>[2x]HMLPKDFQWGFATAAYQIEGAIDKDGRGPSIWDTFCAIPGKIADGTSGVTACDSYNRTAEDIALLKSLGAKSYRFSISWSRIIPKGGRDDPVNQLGIDHYAQFVDDLLEAGITPFITLFHWDLPEELHQRYGGLLNRTEFPLDFENYARVMFKALPKVRNWITFNEPWCSAILGYGSGTFAPGRQS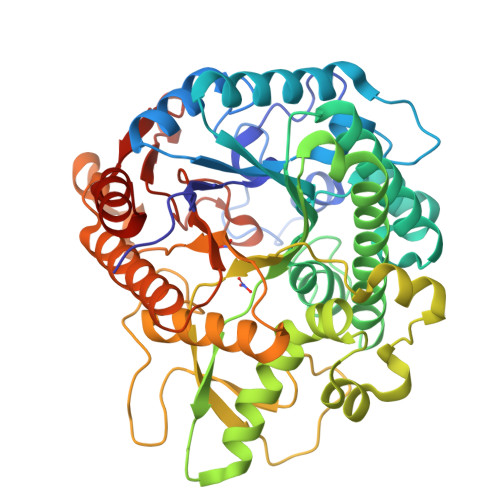TTEPWIVGHNLLVAHGRAVKVYRDEFKDLNDGQIGIVLNGDFTYPWDSSDPLDREAAERRLEFFTAWYADPIYLGDYPASMRKQLGDRLPEFTPEEKAFVLGSNDFYGMNHYTSNYIRHRTSPATADDTVGNVDVLFYNKEGQCIGPETESSWLRPCPAGFRDFLVWISKRYNYPKIYVTENGTSLKGENDLPKEKILEDDFRVNYYNEYIRAMFTAATLDGVNVKGYFAWSLMDNFEWADGYVTRFGVTYVDYENGQQRFPKKSAKSLKPLFDELIAKE>[2x]MALKSLVLLSLLVLVLLLVRVQPSLGKETAAAKFERQ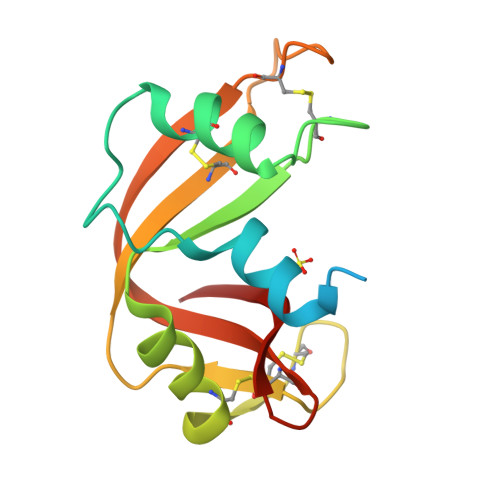HMDSSTSAASSSNYCNQMMKSRNLTKDRCKPVNTFVHESLADVQAVCSQKNVACKNGQTNCYQSYSTMSITDCRETGSSKYPNCAYKTTQANKHIIVACEGNPYVPVHFDASV N-({2-[(6-amino-9H-purin-9-yl)methoxy]ethyl}sulfamoyl)-5-[(3aS,4S,6aR)-2-oxohexahydro-1H-thieno[3,4-d]imidazol-4-yl]pentanamide | C18 H27 N9 O5 S2 | 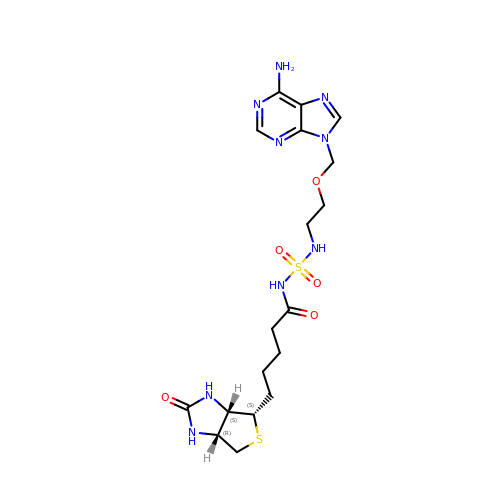HEOBKFIXAMLSMW-OBJOEFQTSA-N(E)-2-(4-chlorophenyl)-N-{(3S)-1-[(2S)-1-(morpholin-4-yl)-1-oxopropan-2-yl]-2-oxopyrrolidin-3-yl}ethenesulfonamide 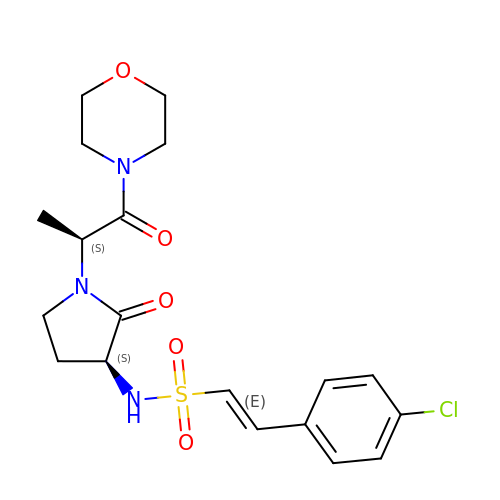| C19 H24 Cl N3 O5 S | DNCVZNVETAOAJO-PPYZAHLJSA-N> GVSKGEELIKEDMHMKLYMEGTVNNHHFKCTSEGEGKPYEGTQTGRIKVVEGGPLPFAFDILATCFMYGSKTFINHTQGIPDFFKQSFPEGFTWERVTTYEDGGVLTATQDTSLQDGC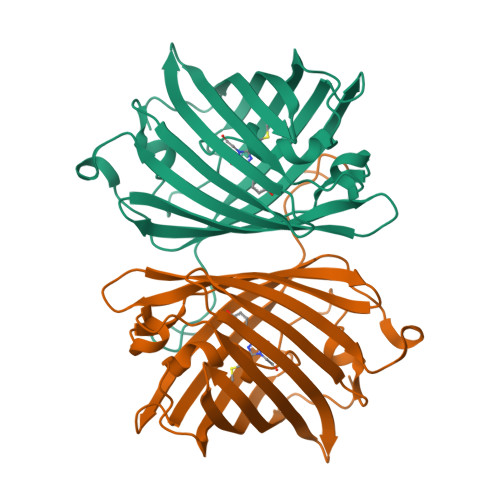LIYNVKIRGVNFPSNGPVMQKKTLGWEASTEMLYPADGGLEGRCDMALKLVGGGHLICNLKTTYRSKKPAKNLKMPGVYFVDRRLERIKEADNETYVEQHEVAVARYCDLPSKLGHKLNGMDELYK> MERITAARGLELRCKGWRQEALLRMLENVLENGENQKELIVYAALAKAARNWPSYHAIVRTLKELEEDETLVIQSGKPIGIFKTHRFAPLIVMANCNLVGRWATSENFYRLQEKGLLIWGGLTAAAWQYIGSQG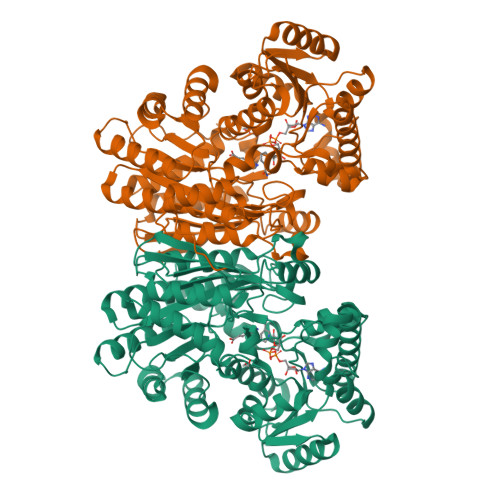VIQGTYEIFQSIARLHFNGSLAGKFILTAGLGGMGGAQPLAGTLAGAAILCVEVSEDRVDRRLQTNYLQRKTRSLDEALLWIEEAVDNLHPVSVGLTGNASDIYPELVRRGITPDIVTDQTSAHDLVYGYVPSGYRVEELEEARANDPEQLQRDAGASIAVEVEAMLELKKRGAIVFDNGNNIRSQAKEYGVQNAFDIDIFTEAFLRPLFARAIGPFRWVALSGELSDIHAIDEFILEAFSDNEVIANWIRLAREHVPVEGLPARIGWFGHGDRTKLALAVNQMVREGKLQGPIAFSRDHLDAASMTHPNIMTERMKDGSDAIADWPLLNAMLNCSSMADLVTIHSGGGGYAGYMTSAGVTLVADGSTESDIRLETTLNNDTGLGVLRYADAGYEESADEVRLKDIRWIKTN> GFPLITITVRGRNVHMKQEHYMKGSDGAPDTGYLWHVPLTFITSKSDMVHRFLLKTKTDVLILPEEVEWIKFNVGMNGYYIVHYEDDGWDSLTGLLKGTHTAVSSNDRASLINNAFQLVSIGKLSIEKALDLSLYLKHETEIMPVFQGLNELIPMYKLMEKRDMNEVETQFKAFLIRLLRDLIDKQTWTDEGSVSERMLRSQLLLLACVHNYQPCVQRAEGYFRKWKESNGNLSLPVDVTLAVFAVGAQSTEGWDFLYSKYQFSLSSTEKSQIEFALCRTQNKEKLQWLLDESFKGDKIKTQEFPQILTLIGRNPVGYPLAWQFL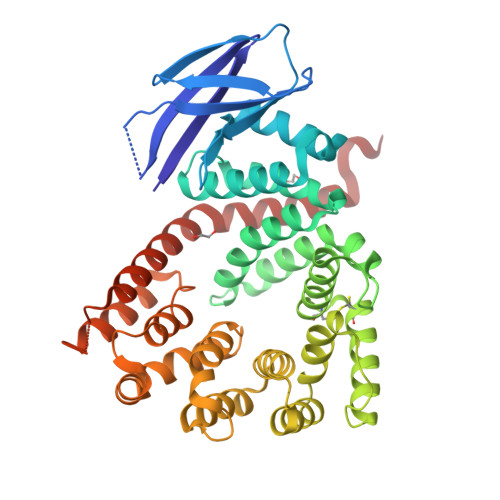RKNWNKLVQKFELGSSSIAHMVMGTTNQFSTRTRLEEVKGFFSSLKENGSQLRCVQQTIETIEENIGWMDKNFDKIRVWLQSEKLERMHHHHHH methyl 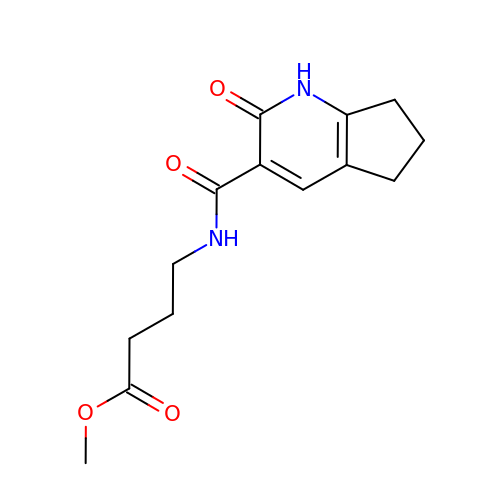4-[(2-oxidanylidene-1,5,6,7-tetrahydrocyclopenta[b]pyridin-3-yl)carbonylamino]butanoate | C14 H18 N2 O4 | LFOKUSURFOQCKJ-UHFFFAOYSA-N>MGSSYHHHHHHSSGENLYFQHMKHGRVFIIKSYSEDDIHRSIKYNIWCSTEHGNKRLDAAYRSMNGKGPVYLLFSVNGSGHFCGVAEMKSAVDYNTCAGVWSQDKW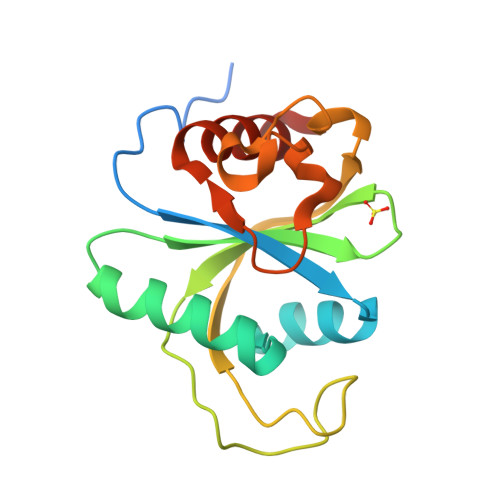KGRFDVRWIFVKDVPNSQLRHIRLENNENKPVTNSRDTQEVPLEKAKQVLKIIASYKHTTS[6x]> GSMDREMILADFQACTGIENIDEAITLLEQ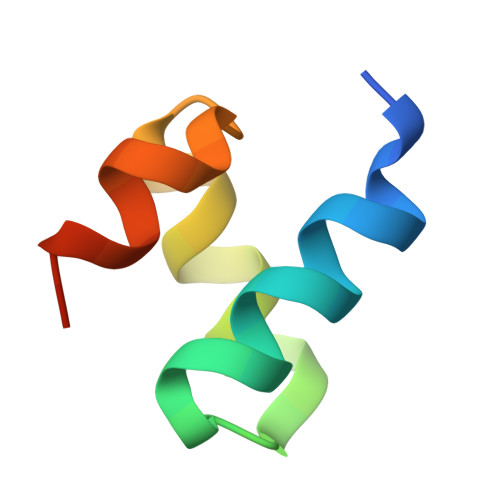NNWDLVAAINGVIPQ RIG-I is an essential innate immune receptor that responds to infection by RNA viruses. The RIG-I signaling cascade is mediated by a series of post-translational modifications, the most important of which is ubiquitination of the RIG-I Caspase Recruitment Domains (CARDs) by E3 ligase Riplet. Riplet is a homodimer composed of an N-terminal RING domain (catalytic domain), CC domain (coiled-coil domain, homodimerization), and C-terminal PrySpry domain (RIG-I recognition domain). Each structure contains two RIG-I molecules, one p3dsRNA24, and one Riplet homodimer, but they differ in the relative positions of two PrySpry domains, which depend on the relative positions of their partner RIG-I molecules.

In the structure containing 23.4% particles, one RIG-I forms a typical end-bound complex with the terminal triphosphate, but the second RIG-I binds to the opposite dsRNA terminus in a “semi-closed” end-bound state, where the CTD has tilted away from its normal orientation while maintaining engagement with the terminal dsRNA diphosphate. This observation is consistent with RIG-I/RNA recognition models in which CTD:RNA interactions are the first point of contact upon RIG-I encounter with RNA, and it provides new insights into the conformational variability of RIG-I CTD complexes. As the second RIG-I in each structure recognizes different types of RNA sites, the two PrySpry domains bind to RIG-I from different approach angles, revealing variable distances between them, ranging from 58 Å to 101 Å. This finding suggests that the CC domains in these complexes are more dynamic than expected (consistent with our inability to visualize them), enabling the complex to accommodate different spacings between sites of PrySpry domains, and enabling PrySpry domains to approach RIG-I Hel2 from different angles. Despite the different relative orientations of PrySpry in the three structures, the PrySpry domain uses the same interface with RIG-I Hel2 in each case. Unfortunately, only the structure of the PrySpry domain of Riplet but not the RING or CC domain could be resolved.

>[2x]MTTEQRRSLQAFQDYIRKTLDPTYILSYMAPWFREEEVQYIQAEKNNKGPMEAATLFLKFLLELQEEGWFRGFLDALDHAGYSGLYEAIESWDFKKIEKLEEYRLLLKRLQPEFKTRIIPTDIISDLSECLINQECEEILQICSTKGMMAGAEKLVECLLRSDKENWPKTLKLALEKERNKFSELWIVEKGIKDVETEDLEDKMETSDIQIFYQEDPECQNLSENSCPPSEVSDTNLYSPFKPRNYQLELALPAMKGKNTIICAPTGCGKTFVSLLICEHHLKKFPQGQKGKVVFFANQIPVYEQQKSVFSKYFERHGYRVTGISGATAENVPVEQIVENNDIIILTPQILVNNLKKGTIPSLSIFTLMIFDECHNTSKQHPYNMIMFNYLDQKLGGSSGPLPQVIGLTASVGVGDAKNTDEALDYICKLCASLDASVIATVKHNLEELEQVVYKPQKFFRKVESRISDKFKYIIAQLMRDTESLAKRICKDLENLSQIQNREFGTQKYEQWIVTVQKACMVFQMPDKDEESRICKALFLYTSHLRKYNDALIISEHARMKDALDYLKDFFSNVRAAGFDEIEQDLTQRFEEKLQELESVSRDPSNENPKLEDLCFILQEEYHLNPETITILFVKTRALVDALKNWIEGNPKLSFLKPGILTGRGKTNQNTGMTLPAQKCILDAFKASGDHNILIATSVADEGIDIAQCNLVILYEYVGNVIKMIQTRGRGRARGSKCFLLTSNAGVIEKEQINMYKEKMMNDSILRLQTWDEAVFREKILHIQTHEKFIRDSQEKPKPVPDKENKKLLCRKCKALACYTADVRVIEECHYTVLGDAFKECFVSRPHPKPKQFSSFEKRAKIFCARQNCSHDWGIHVKYKTFEIPVIKIESFVVEDIATGVQTLYSKWKDFHFEKIPFDPAEMSK;>[2x]MAGLGLGSAVPVWLAEDDLGCIICQGLLDWPATLPCGHSFCRHCLEALWGARDARRWACPTCRQGAAQQPHLRKNTLLQDLADKYRRAAREIQAGSDPAHCPCPGSSSLSSAAARPRRRPELQRVAVEKSITEVAQELTELVEHLVDIVRSLQNQRPLSESGPDNELSILGKAFSSGVDLSMASPKLVTSDTAAGKIRDILHDLEEIQEKLQESVTWKEAPEAQMQGELLEAPSSSSCPLPDQSHPALRRASRFAQWAIHPTFNLKSLSCSLEVSKDSRTVTVSHRPQPYRWSCERFSTSQVLCSQALSSGKHYWEVDTRNCSHWAVGVASWEMSRDQVLGRTMDSCCVEWKGTSQLSAWHMVKETVLGSDRPGVVGIWLNLEEGKLAFYSVDNQEKLLYECTISASSPLYPAFWLYGLHPGNYLIIKQVKV>[3x]MDFSRNLYDIGEQLDSEDLASLKFLSLDYIPQRKQEPIKDALMLFQRLQEKRMLEESNLSFLKELLFRINRLDLLITYLNTRKEEMERELQTPGRAQISAYRVMLYQISEEVSRSELRSFKGGLQEEISKCKLDDDMNLLDIFIEMEKRVILGEGKLDILKRVCAQINKSLLKIINDYEEFSKERSSSLEGSPDEFSNGEELCGVMTISDSPREQDSESQTLDKVYQMKSKPRGYCLIINNHNFAKAREKVPKLHSIRDRNGTHLDAGALTTTFEELHFEIKPHDDCTVEQIYEILKIYQLMDHSNMDCFICCILSHGDKGIIYGTDGQEAPIYELTSQFTGLKCPSLAGKPKVFFIQAAQGDNYQKGIPVETASEEQPYLEMALSSPQTRYIPDEADFLLGMATVNNCVSYRNPAEGTWYIQSLCQSLRERCPRGDDILTILTEVNYEVSNKDDKKNMGKQMPQPTFTLRKKLVFPSD;>[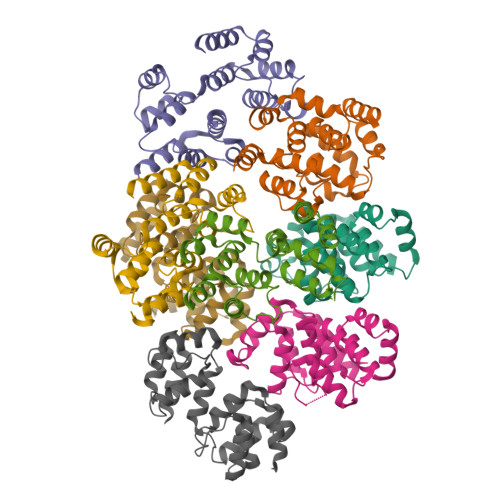5x]MSAEVIHQVEEALDTDEKEMLLFLCRDVAIDVVPPNVRDLLDILRERGKLSVGDLAELLYRVRRFDLLKRILKMDRKAVETHLLRNPHLVSDYRVLMAEIGEDLDKSDVSSLIFLMKDYMGRGKISKEKSFLDLVVELEKLNLVAPDQLDLLEKCLKNIHRIDLKTKIQKYKQSVQGAGTS> SEPPLHDFYCSRLLDLVFLLDGSSRLSEAEFEVLKAFVVDMMERLRVSQKWVRVAVVEYHDGSHAYIGLKDRKRPSELRRIASQVKYAGSQVASTSEVLKYTLFQIFSKIDRPEASRIALLLMASQEPQRM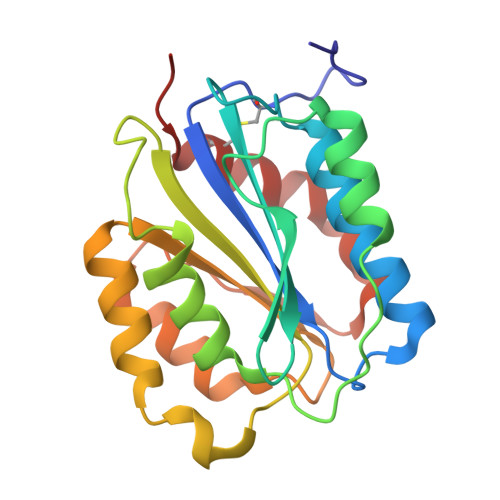SRNFVRYVQGLKKKKVIVIPVGIGPHANLKQIRLIEKQAPENKAFVLSSVDELEQQRDEIVSYLCDLAPEA>MGHHHHHHMIEENLKQKIHDKFVAAKKNGHLKVTHAESKKLKDPQTTTQYWVTFAPSLALKPDANK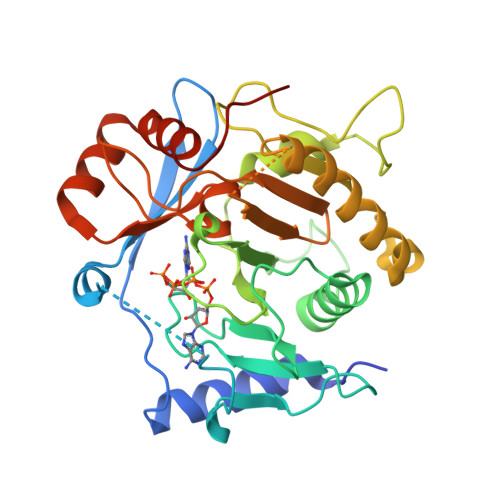NSDSKAEDPFANPDEELVVTEDLNGDGEYKLLLNKFPVVPEHSLLVTSEFKDQRSALTPSDLMTAYNVLCSLQGDKDDDVTCERYLVFYNCGPHSGSSQDHKALQIMQMPEKFIPFQDVLCNGKDHFLPTFNAEPLQDDKVSFAHFVLPLPESSDQVDEDLLAMCYVSLMQRALTFFQDWTNESPELTKSYNVLLTKKWICVVPRSHAKSGPPLMLNINSTGYCGMILVKDREKLENLTEDPHLVDKSLLQCGFPNTAGQKPTEYHY[2x]>MAREVKLTKAGYERLMQQLERERERLQEATKILQELMESSDDYDDSGLEAAKQEKARIEARIDSLEDILSRAVILEEGSGEVIGLGSVVELEDPLSGERLSVQVVSPAEANVLD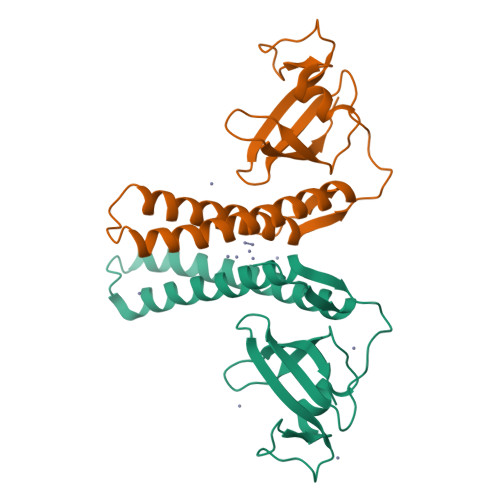TPMKISDASPMGKALLGHRVGDVLSLDTPKGRREFRVVAIHG[4x]>[2x]QTKADVVWKDVDGVSMPIPPKTHPRLYLREQQVPDLKNRMNDPKLKKVWADMIKMQEDWKPADIPEVKDFRFYFNQKGLTVRVELMALNYLMTKDPKVGREAITSIIDTLETATFKP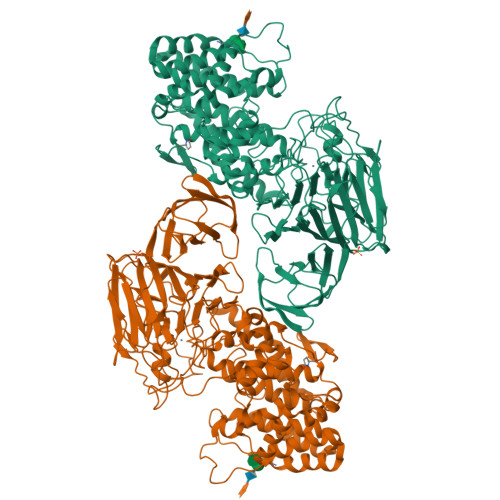AGDISRGIGLFMVTGAIVYDWCYDQLKPEEKTRFVKAFVRLAKMLECGYPPVKDKSIVGHASEWMIMRDLLSVGIAIYDEFPEMYNLAAGRFFKEHLVARNWFYPSHNYHQGMSYLNVRFTNDLFALWILDRMGAGNVFNPGQQFILYDAIYKRRPDGQILAGGDVDYSRKKPKYYTMPALLAGSYYKDEYLNYEFLKDPNVEPHCKLFEFLWRDTQLGSRKPDDLPLSRYSGSPFGWMIARTGWGPESVIAEMKVNEYSFLNHQHQDAGAFQIYYKGPLAIDAGSYTGSSGGYNSPHNKNFFKRTIAHNSLLIYDPKETFSSSGYGGSDHTDFAANDGGQRLPGKGWIAPRDLKEMLAGDFRTGKILAQGFGPDNQTPDYTYLKGDITAAYSAKVKEVKRSFLFLNLKDAKVPAAMIVFDKVVASNPDFKKFWLLHSIEQPEIKGNQITIKRTKNGDSGMLVNTALLPDAANSNITSIGGKGKDFWVFGTNYTNDPKPGTDEALERGEWRVEITPKKAAAEDYYLNVIQIADNTQQKLHEVKRIDGDKVVGVQLADRIVTFSKTSETVDRPFGFSVVGKGTFKFVMTDLLPGTWQVLKDGKILYPALSAKGDDGALYFEGTEGTYRFLR3-ethyl-1,3-diazatricyclo[6.3.1.0^{4,12}]dodeca-4,6,8(12)-trien-2-imine 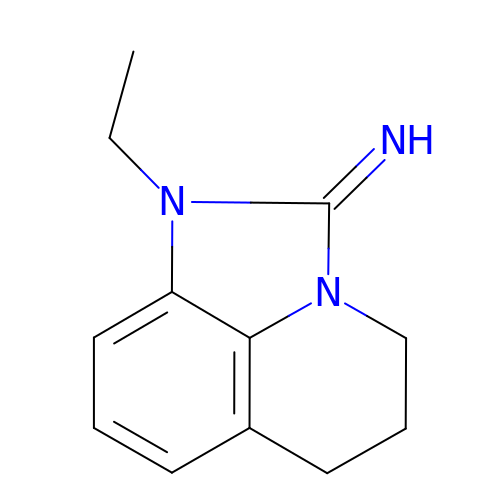| C12 H15 N3 | PBCCOMRKDASFBZ-OUKQBFOZSA-N The plasma membrane of fungal and plant cells contains a proton-pumping P-type adenosine triphosphatase (ATPase) that maintains the intracellular pH and generates a proton-motive force, driving the import of nutrients by secondary transporters. Unlike any other known P-type ATPase, Pma1 is a hexamer that localizes to specific ordered microdomains in the fungal plasma membrane. Autoinhibited Pma1 hexamers in the plasma membrane of starving fungi are activated by glucose signaling and subsequent phosphorylation of the autoinhibitory domain. We have determined the structure of hexameric Pma1 from Neurospora crassa by electron cryo-microscopy at 3.3-Å resolution, elucidating the molecular basis for hexamer formation and autoinhibition and providing a basis for structure-based drug development.

We collected single-particle cryo-EM data of the hexameric form of Pma1 from Neurospora crassa plasma membrane in its autoinhibited state and obtained a hexamer map at 3.28-Å resolution. The Pma1 hexamer forms a ring with sixfold symmetry, with a maximum outer diameter of 167 Å and an inner cavity measuring 24 to 55 Å in diameter in the cytosolic and transmembrane regions, respectively. Monomer contacts are mediated by both the cytosolic domains and the transmembrane domains. Specifically, there are two connections between the cytosolic domains: a loose contact between the conserved Thr-Gly-Glu-Ser (TGES) loop in the A domain (residues 231 to 235) and two α-helix termini in the P domain (Tyr541, Arg570, and Gln571). The second, more extensive contact between the P domains of adjacent monomers is mediated entirely via the autoinhibitory R domain (and see further discussion below). The interactions in the transmembrane region involve residues in M3 of one monomer, and M7 and M10 of the adjacent monomer, augmented by two polar contacts from Ser316 and Asn317 in L3-L4 to Gln780 (M7) and Arg859 (M10). The R domains are closely sandwiched between adjacent P domains, forming an extensive interaction network. R domains of adjacent monomers interact directly: Ser892 and Pro893 interact with Leu902 of the adjacent R helix, thereby linking all R domains within the hexamer. Opposite this dip, on the inside of the ring, the cytosolic membrane surface bulges upward toward the P domain, probably attracted by the partial positive charge at the N-terminal end of M3 and by Lys749 in the L6-L7 loop. Both the “dip” and the “bulge” are also evident from the cryo-EM map of the micelle surrounding the Pma1 hexamer particles [likely consisting of a mixture of β-dodecyl-maltopyranoside (DDM) with residual membrane lipids]. We find no structural basis for cooperativity between the monomers in the hexamer, but the structure implies that autoinhibition is enhanced by—if not dependent on—a hexamer context.

>[6x]MADHSASGAPALSTNIESGKFDEKAAEAAAYQPKPKVEDDEDEDIDALIEDLESHDGHDAEEEEEEATPGGGRVVPEDMLQTDTRVGLTSEEVVQRRRKYGLNQMKEEKENHFLKFLGFFVGPIQFVMEGAAVLAAGLEDWVDFGVICGLLLLNAVVGFVQEFQAGSIVDELKKTLALKAVVLRDGTLKEIEAPEVVPGDILQVEEGTIIPADGRIVTDDAFLQVDQSALTGESLAVDKHKGDQVFASSAVKRGEAFVVITATGDNTFVGRAAALVNAASGGSGHFTEVLNGIGTILLILVIFTLLIVWVSSFYRSNPIVQILEFTLAITIIGVPVGLPAVVTTTMAVGAAYLAKKKAIVQKLSAIESLAGVEILCSDKTGTLTKNKLSLHDPYTVAGVDPEDLMLTACLAASRKKKGIDAIDKAFLKSLKYYPRAKSVLSKYKVLQFHPFDPVSKKVVAVVESPQGERITCVKGAPLFVLKTVEEDHPIPEEVDQAYKNKVAEFATRGFRSLGVARKRGEGSWEILGIMPCMDPPRHDTYKTVCEAKTLGLSIKMLTGDAVGIARETSRQLGLGTNIYNAERLGLGGGGDMPGSEVYDFVEAADGFAEVFPQHKYNVVEILQQRGYLVAMTGDGVNDAPSLKKADTGIAVEGSSDAARSAADIVFLAPGLGAIIDALKTSRQIFHRMYAYVVYRIALSIHLEIFLGLWIAILNRSLNIELVVFIAIFADVATLAIAYDNAPYSQTPVKWNLPKLWGMSVLLGVVLAVGTWITVTTMYAQGENGGIVQNFGNMDEVLFLQISLTENWLIFITRANGPFWSSIPSWQLSGAIFLVDILATCFTIWGWFEHSDTSIVAVVRIWIFSFGIFCIMGGVYYILQDSVGFDNLMHGKSPKGNQKQRSLEDFVVSLQRVSTQHEKSQ2',5'-dideoxy-5'-[(diphenylmethyl)(methyl)amino]uridine 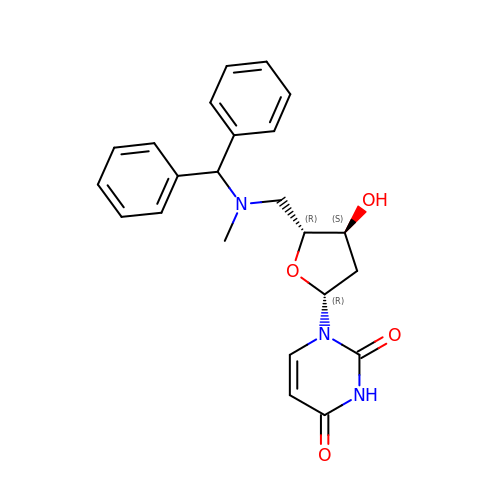| C23 H25 N3 O4 | GMULPQZINUAVEX-QKNQBKEWSA-N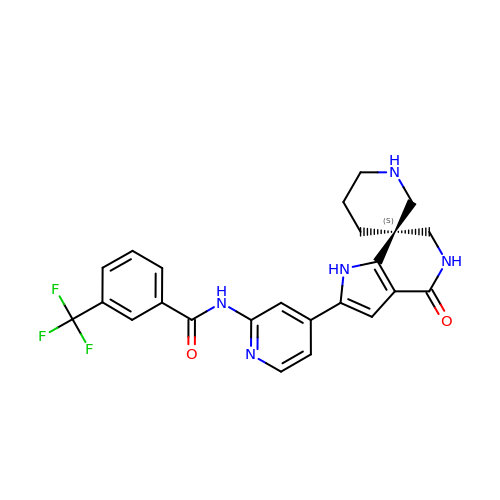N-{4-[(3S)-4'-oxo-1',4',5',6'-tetrahydrospiro[piperidine-3,7'-pyrrolo[3,2-c]pyridin]-2'-yl]pyridin-2-yl}-3-(trifluoromethyl)benzamide | C24 H22 F3 N5 O2 | FEVPBNYNYKIJAR-QHCPKHFHSA-N>[6x]MHHHHHHGSMSNEQTFIAIKPDGVQRGLIGPIISRFENRGFKLVAMKLVSPPQSQLEQHYADLSDKPFFKGLVSYMLSGPICAMVWEGR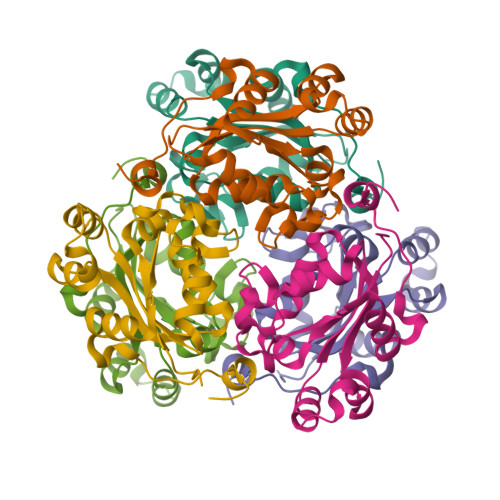DVVKTGRTILGATNPLASAPGTIRGDFAIDVGRNVCHGSDSVENAKKEIALWFKPEELISWKSATFDWVYEKA>[2x]MSTRKAVIGYYFIPTNQINNYTETDTSVVPFPVSNITPAKAKQLTHIN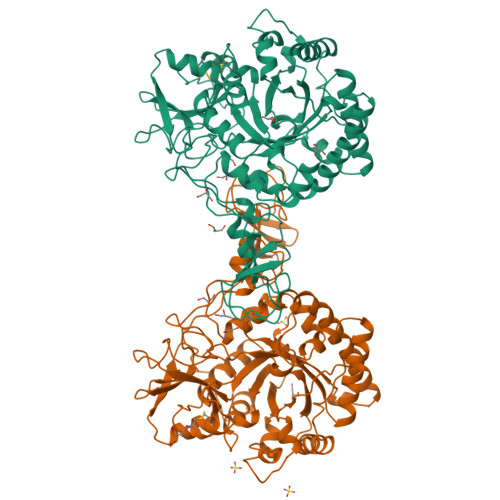FSFLDINSNLECAWDPATNDAKARDVVNRLTALKAHNPSLRIMFSIGGWYYSNDLGVSHANYVNAVKTPASRAKFAQSCVRIMKDYGFDGVNIDWEYPQAAEVDGFIAALQEIRTLLNQQTITDGRQALPYQLTIAGAGGAFFLSRYYSKLAQIVAPLDYINLMTYDLAGPWEKVTNHQAALFGDAAGPTFYNALREANLGWSWEELTRAFPSPFSLTVDAAVQQHLMMEGVPSAKIVMGVPFYGRAFKGVSGGNGGQYSSHSTPGEDPYPSTDYWLVGCEECVRDKDPRIASYRQLEQMLQGNYGYQRLWNDKTKTPYLYHAQNGLFVTYDDAESFKYKAKYIKQQQLGGVMFWHLGQDNRNGDLLAALDRYFNAADYDDSQLDMGTGLRYTGVGPGNLPIMTAPAYVPGTTYAQGALVSYQGYVWQTKWGYITSAPGSDSAWLKVGRVA>[3x]PLRMGGNGQLQYWPFSSSDLYNWKNNNPSFSEDPGKLTALIESVLTTHQPTWDDCQQLLGTLLTGEEKQRVLLEARKAVRGNDGRPTQLPNEVDAAFPLERPDWDYTTQRGR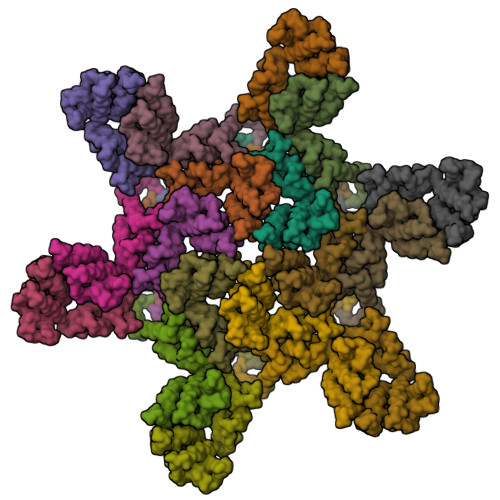NHLVLYRQLLLAGMQNAGRSPTNLAKVKGITQGPNESPSAFLERLKEAYRRYTPYDPEDPGQETNVSMSFIWQSAPDIGRKLERLEDLKSKTLGDLVREAEKIFNKRETPEEREERIRRETEEK> LKLCSPEEFTRLCREKTQEIYPIKEANGRTRKALIICNTEFKHLSLRYGANFDIIGMKGLLEDLGYDVVVKEELTAEGMESEMKDFAALSEHQTSDSTFLVLMSHGTLHGICGTMHSEKTPDVLQYDTIYQIFNNCHCPGLRDKPKVIIVQAARGGNSGEMWIR;> VKLSHVEKDFIAFYSTTPHHLSYRDKTGGSYFITRLISCFRKHACSCHLFDIFLKVQQSFEKASIHSQMPTIDRATLTRYFYLFPGN;> FTRLCREKTQEIYPIKEANGRTRKALIICNTEFKHLSLRYGANFDIIGMKGLLEDLGYDVVVKEELTAEGMESEMKDFAALSEHQTSDSTFLVLMSHGTLHGICGTMHSEKTPDVLQYDTIYQIFNNCHCPGLRDKPKVIIVQAARGGNSGEMWI;> AVKLSHVEKDFIAFYSTTPHHLSYRDKTGGSYFITRLISCFRKHACSCHLFDIFLKVQQS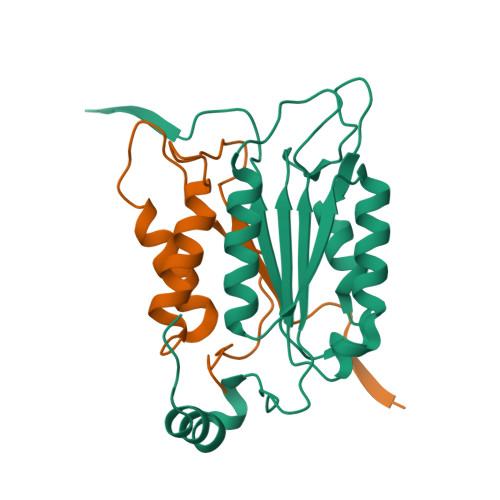FEKASIHSQMPTIDRATLTRYFYLFPGN>[6x]MAELRSFIFIDRLQPQTMSYLGTWIKGALPRANMAAQIIEVAPGLDIEGVTDVALKHAEVK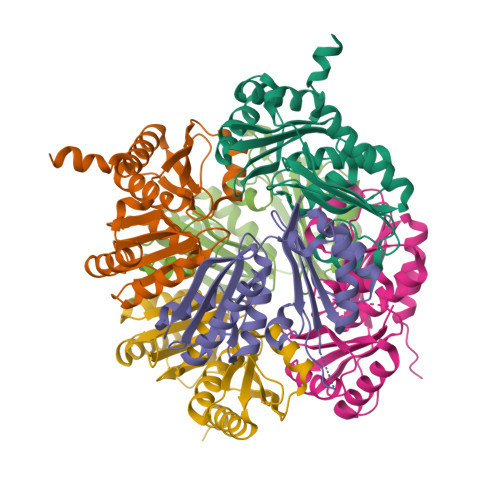AGILVVERQFGYLEFHGETGAVKAAADAALDYLGGDPDAAVRPEILASRIISSIDHQHAFLINRNKIGSMVLPGESLFVLEVAPASYAILATNEAEKAADVKVVDFRMIGATGRVYLSGTEADVRQAADAARDALAVLQGAKLAAALEHHHHHH> SLNPRDVVIVDFGRTPMGRSKGGMHRNTRAEDMSAHLISKVLERNSKVDPGEVEDVIWGCVNQTLEQGWNIARMASLMTQIPHTSAAQTVSRLCGSSMSALHTAAQAIMTGNGDVFVVGGVEHMGHVSMMHGVDPNPHMSLYAAKASGMMGLTAEMLGKMHGISREQQDAFAVRSHQLAHKATVEGKFKDEIIPMQGYDENGFLKIFDYDETIRPDTTLESLAALKPAFNPKGGTVTAGTSSQITDGASCMIVMSAQRAKDLGLEPLAVIRSMAVAGVDPAIMGYGPVPATQKALKRAGLNMADIDFIELNEAFAAQALPVLKDLKVLDKMNEKVNLHGGAIALGHPFGCSGARISGTLLNVMKQNGGTFGLSTMCIGLGQGIATVFER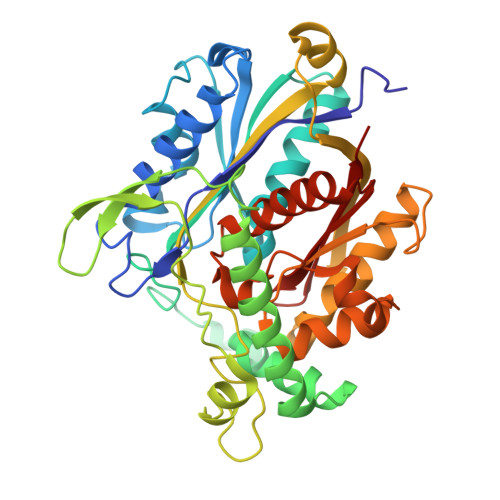V> MHHHHHHLILAPMVRVGTLPMRLLALDYGADIVYCEELIDLKMIQCKRVVNEVLSTVDFVAPDDRVVFRTCEREQNRVVFQMGTSDAERALAVARLVENDVAGIDVNMGCPKQYSTKGGMGAALLSDPDKIEKILSTLVKGTRRPVTCKIRILPSLEDTLSLVKRIERTGIAAIAVHGRKREERPQHPVSCEVIKAIADTLSIPVIANGGSHDHIQQYSDIEDFRQATAASSVMVARAAMWNPSIFLKEGLRPLEEVMQKYIRYAVQYDNHYTNTKYCLCQMLREQLESPQGRLLHAAQSSREICEAFGLGAFYEETTQELDAQQAR

The genes encoding dihydrouridine synthases (Dus) have been identified in yeast Saccharomyces cerevisiae and Escherichia coli. These enzymes are homologous to dihydroorotate dehydrogenases and dihydropyrimidine dehydrogenases and they use a flavin mononucleotide (FMN) to catalyze hydride transfer from NAD(P)H to the uridine substrate. The human enzyme conserves the ‘bona fide’ Dus domain that spans the first 330 amino acids, while a presumably unstructured linker (residues 331–367) connects the latter to an unprecedented double-stranded RNA binding domain (dsRBD) formed by residues 368 to 433. Using biochemical analysis and structural characterization, we here show that HsDus2 uses a unique strategy for binding and modifying its tRNA substrate. In contrast to other Dus proteins, HsDus2 has a dsRBD, which is the primary tRNA binding site.

HsDus2dusD crystallized in the space group I222 with one molecule in the asymmetric unit.The structure confirmed the monomeric state of the domain observed by gel filtration. The structure of HsDus2dusD is organized into two distinct sub-domains. The N-terminal region consists of a α8/β11 TIM barrel fold, in which a central barrel composed of eight parallel beta strands is surrounded by 8 alpha helices. As expected for flavoenzymes with α/β barrels, a well-defined electron density, assigned to the redox FMN cofactor, lies at the center of the β barrel structure close to the C-terminal end of barrel-forming strands with the re-face of the isoalloxazine ring oriented towards the barrel. Remarkably, the TIM barrel core diverges from the classical α8/β8 fold because three additional β strands inserted between Lys53 and Thr76 form a new antiparallel β sheet (β3−β5), a feature not observed in the other Dus structures. The helical sub-domain is formed by a 5-helix bundle that caps the top of the FMN binding site, while it is composed of four helices in the other known Dus structures. A consequence of this additional helix is that the C-terminus borne by helix α13 points toward the opposite direction compared to the other Dus, thereby orienting the dsRDB domain. Remarkably, this domain displays a less positively charged surface of the helical sub-domain of HsDus2 compared to its known Dus counterparts, which could explain why HsDus2dusD exhibit a weak tRNA binding. In contrast to other structurally characterized Dus proteins, in which the isoalloxazine ring is planar, the electron density of the FMN cofactor in HsDus2dusD revealed a ‘butterfly’ bending at the N(5)–N(10) hinge, with the concave side corresponding to the re-face of the ring. Since the oxidized flavin ring system is widely described to be planar, while bending along the N(5)–N(10) axis occurs only upon reduction of the isoalloxazine ring, the FMN cofactor of HsDus2dusD was likely reduced by the X-ray beam during data collection.>[2x]AAPTATVTPSSGLSDGTVVKVAGAGLQAGTAYWVAQ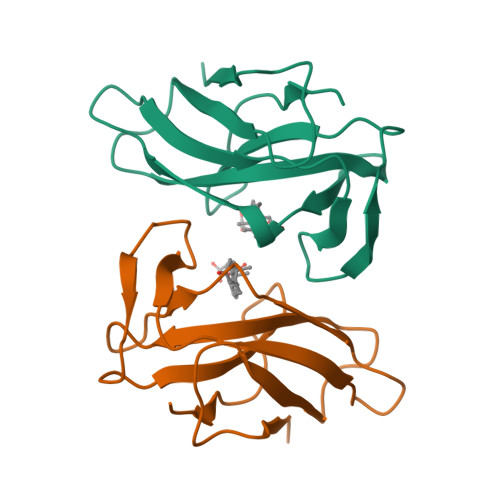SAWVDTGVYASNPADISSVTADANGSASTSLTVRRSFEGFLWDGTRWGTVDCTTAACHVTLRDALSNGPEGVAISF>[2x]MRGSHHHHHHGSMTDTYLHETLVFDNKLSYIDNQRDTD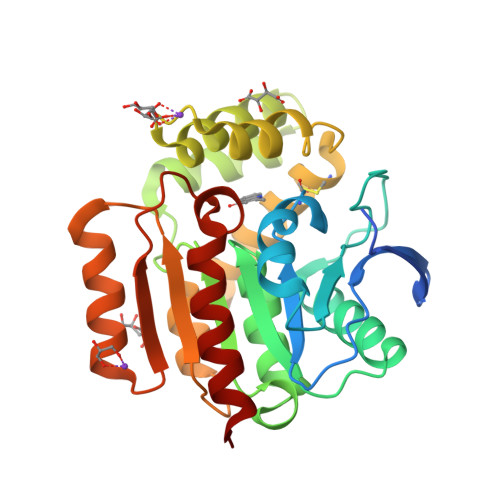GPAILLLPGWCHDHRVYKYLIQELDADFRVIVPNWRGHGLSPSEVPDFGYQEQVKDALEILDQLGVETFLPVSHSHGGWVLVELLEQAGPERAPRGIIMDWLMWAPKPDFAKSLTLLKDPERWREGTHGLFDVWLDGHDEKRVRHHLLEEMADYGYDCWGRSGRVIEDAYGRNGSPMQMMANLTKTRPIRHIFSQPTEPEYEKINSDFAEQHPWFSYAKLGGPTAFPAIDVPDRAAVHIREFATAIRQGQ> STEIPSLSASYANSFKIGAAVHTRMLQTEGEFIAKHYNSVTAENQMKFEEVHPREHEYTFEAADEIVDFAVARGIGVRGHTLVWHNQ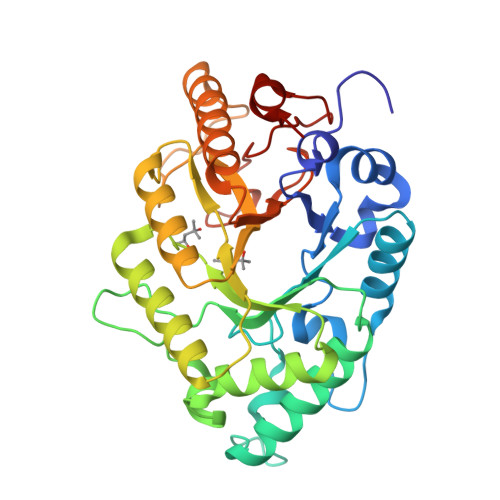TPAWMFEDASGGTASREMMLSRLKQHIDTVVGRYKDQIYAWDVVNEAIEDKTDLIMRDTKWLRLLGEDYLVQAFNMAHEADPNALLFYNDYNETDPVKREKIYNLVRSLLDQGAPVHGIGMQGHWNIHGPSMDEIRQAIERYASLDVQLHVTELDLSVFRHEDQRTDLTEPTAEMAELQQKRYEDIFGLFREYRSNITSVTFWGVADNYTWLDNFPVRGRKNWPFVFDTELQPKDSFWRIIGQD> SNAVGKQSPANPAPSRPLNDYVGVYANDYWGPATVTYHDGQLRLSLGPKNQTFDLTHWD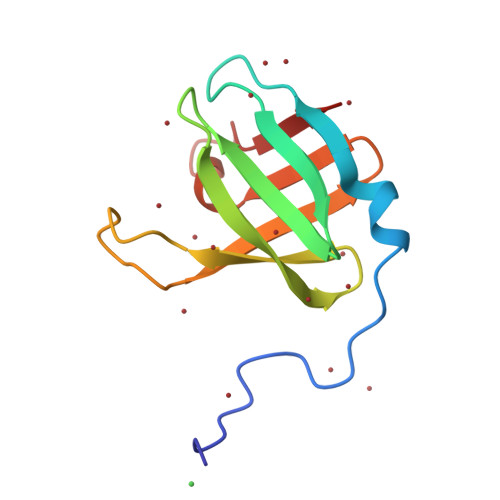GDTFTFTLSTENALPGSISKATFAGDTLNLEYYDADKLGTFTR Adenovirus-derived nanoparticles (ADDomer) comprise 60 copies of adenovirus penton base protein (PBP). In the ADDomer, the PBP monomers spontaneously assembles to form a pentamer, and twelve pentamers organize into a dodecamer characterized by high stability and thermotolerance exceeding 50°C.16–18 The PBP monomer folds into two distinctive domains; the jelly-roll fold domain which is located in the core of the dodecamer and assumed to be responsible for multimerization, and a solvent-facing exterior domain, called the crown domain. The crown domain comprises two highly flexible regions, called variable loop (VL) and arginine-glycine-aspartic acid (RGD) motif-containing loop. To expand the scope of ADDomers for new applications, we engineered ADDobodies, representing PBP crown domain, genetically separated from PBP multimerization domain.

To validate our design by high-resolution structural analysis using X-ray crystallography, we created an ADDobody prototype with minimized loops, called ADDobody-Xtal, based on the assumption that long flexible loops could be detrimental to crystal lattice formation. During X-ray diffraction data collection and structure determination, two different crystal forms were observed: In the absence of zinc ions, ADDobody crystals adopted space group P1 and diffracted to a resolution of 3.17 Å. In the zinc-free ADDobody crystal form, the VL loop could be manually traced through the density in some of the monomers. In the zinc-free ADDobody crystal form, twenty ADDobody monomers are found in the asymmetric unit. Of note, five ADDobody monomers formed a penton in the crystal reminiscent of the ring-like arrangement in pentons formed by the PBP in the ADDomer. Two such penton rings in the zinc-free triclinic crystal form a barrel-like decamer where the VL and RGD loops are outward facing and accessible. The Coulomb potential indicates a complementary patch of negative and positive charges at the ADDobody surface which contribute to penton ring formation in the crystals. Specifically, D106 forms a charge-charge interaction with R83. The stacking of the two penton rings is mostly mediated by van der Waals interactions, with residue F153 playing a central role. A cation-V interaction is formed between F153 and R140 of an adjacent chain, and F16 could also interact with F153 of the neighboring ADDobody polypeptide chain.

>[20x]GAMGSGIQPNVNEYMFSNKFKARVMVSRKAPEGVTVNDTYDHKEDILKYEWFEFILPEGNFSATMTIDLMNNAIIDNYLEIGRQNGVLESDIGVKFDTRNFRLGWDPETKLIMPGVYTYEAFHPDIVLLPGCGVDFTESRLSNLLGIRKRHPFQEGFKIMYEDLEGGNIPALLDVTAYEESKKDTTTETTTKKELKIQPLEKDSKSRSYNVLEDKINTAYRSWYLSYNYGNPEKGIRSWTLLTTSDVTCGANGDSGNPVFSKSFYNEQAVYSQQLRQATSLTHVFNRFPENQILIRPPAPTITTVSENVP> MDNHSSVPWASAASVTCLSLDAKCHSSSSSSSSKSAASSISAIPQEETQTMRHIAHTQRCLSRLTSLVALLLIVLPMVFSPAHSCGPGRGLGRHRARNLYPLVLKQTIPNLSEYTNSASGPLEGVIRRDSPKFKDLVPNYNRDILFRDEEGTGADRLMSKRCKEKLNVLAYSVMNEWPGIRLLVTESWDEDYHHGQESLHYEGRAVTIATSDRDQSKYGMLARLAVEAGFDWVSYVSRRHIYCSVKSDSSISSHVHGCFTPESTALLESGVRKPLGELSIGDRVLSMTANGQAVYSEVILFMDRNLEQMQNFVQLHTDGGAVLTVTPAHLVSVWQPESQKLTF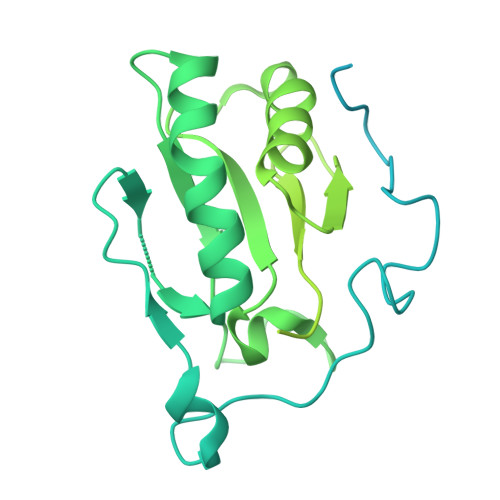VFADRIEEKNQVLVRDVETGELRPQRVVKVGSVRSKGVVAPLTREGTIVVNSVAASCYAVINSQSLAHWGLAPMRLLSTLEAWLPAKEQLHSSPKVVSSAQQQNGIHWYANALYKVKDYVLPQSWRHD> MTSKDHVKSQIPRLSAINDLHKIWPTVEEHGAAIIESFLSLDIVRRLNEEVDPFVKIEPIPAAKTKDHPNHVLSTTTRLVNVLAPISKAYREDVLNSKVLHRICSDAFHVYGDYWVLMGAVMELAPSNPAQPLHRDMRFSHPIVEYLKPDAPATSINFLVALS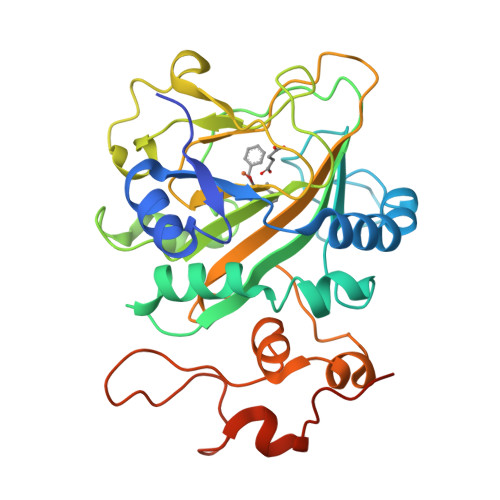PFTAENGATHVILGSHKWQNLSNVSMDATVRALMNPGDALLITDSTIHCGGAETTGTETRRLLTITMGISQLTPLESNLAVPRPVIESLTPLAQRLLGWASQRSAAPRDIGLLTIRGNSIEKTMNLKAEQPLHDDEAEPLCRETI> SGSLNIG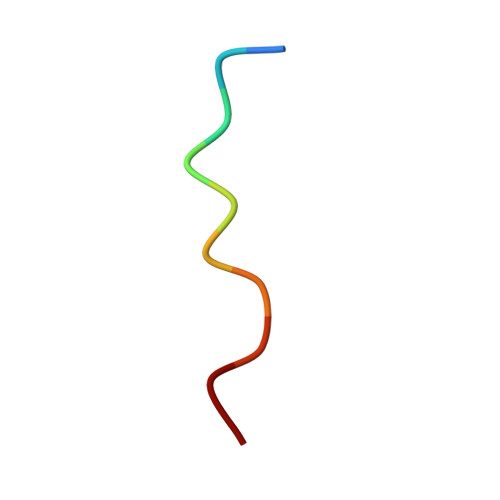SLK> MGSDKIHHHHHHMKKEKVEERIREILRPGWDLLTEEAMLYSATVGGKRIRPLLVLTLGEDLGVE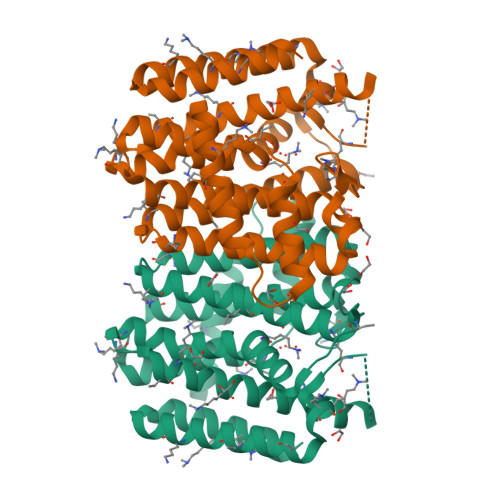EEKLLDVAVAVELFHTASLIHDDLPPIDNADFRRGKPSCHRTYGEDIALLAGDGLFFLAFSQISKIGNSKIFEEFSETAYKLLLGEAMDVEFERRKMEVSQEMVERMYAFKTGALFAFCFSAPFILKGKDHTKMKLLGEKFGVAFQIYDDLKDILGSFEKVGKDLGKDTEKVTLVKKVGIQKAREMADKYYEEVLKGIESEGLFRTLFLLKELKQMVEER> MGSSHHHHHHSQGSMSLVGSNLHVFTIAELRAVTRDFSMTNFIGEGGFGPVYKGYVHDKTKPGLAAQTVAVKLLDLEGGQGHTEWQTEVFFLGQLRHPHLVKLIGYCYEDEHRLLVYEFMTRGSLEKHLFKKYAASLPWSTRLKIAIGAAKGLAFLHEAEKPVIYRDFKTSNILLDSDYKAKLSDFGLAKDGPEDDETHVAARVMGTQGYAAPEYIMTGHLTAKSDVYGYGVVLLELLSGRKAVDKTRPPREQSLVEWARPYLTDARRLDRVMDPSLAGQYSTRAAHKAAAVAHQCVALNPKSRPHMSAVVDALEPLLALDDCIVG

We identified ScRIPK, a member of the RLCK VII subfamily, by a screen for sugarcane orthologs of Arabidopsis RIPK and rice GUDK. Thus, ScRIPK is a member of the RLCK VII subfamily localized in the plasma membrane. Furthermore, bacterial growth was measured to determine the bacterial proliferation inside plants, showing that transgenic plants exhibited significantly higher bacterial proliferation than that in wild-type plants at 3 days. These results suggest that ScRIPK plays role in regulating drought tolerance and disease defense in Arabidopsis. Like the typical structure of protein kinases, ScRIPK-KD contains a small N-lobe, composed of five β-sheets and an α-helix, and a large C-lobe, composed of six helices, an activation loop, and a catalytic loop.

We also analyzed the ScRIPK-KD activation loopresidues that mediated the kinase functions. This activation loop contains three phosphorylation sites, namely, T250, S253, and T254, as indicated by the electron density.> MDFGSLETVVANSAFIAARGSF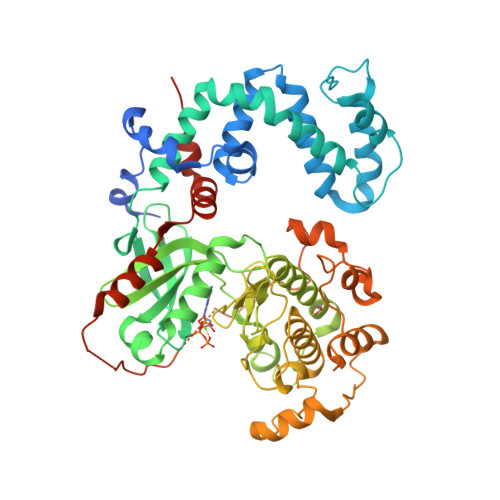DASSGPASRDRKYLARLKLPPLSKCEALRESLDLGFEGMCLEQPIGKRLFQQFLRTHEQHGPALQLWKDIEDYDTADDALRPQKAQALRAAYLEPQAQLFCSFLDAETVARARAGAGDGLFQPLLRAVLAHLGQAPFQEFLDSKYFLRFLQWKWLEAQPMGEDWFLDFRVLGRGGFGEVFACQMKATGKLYACKKLNKKRLKKRKGYQGAMVEKKILAKVHSRFIVSLAYAFETKTDLCLVMTIMNGGDIRYHIYNVDEDNPGFQEPRAIFYTAQIVSGLEHLHQRNIIYRDLKPENVLLDDDGNVRISDLGLAVELKAGQTKTKGYAGTPGFMAPELLLGEEYDFSVDYFALGVTLYEMIAARGPFRARGEKVENKELKQRVLEQAVTYPDKFSPASKDFCEALLQKDPEKRLGFRDGSCDGLRTHPLFRDISWRQLEAGMLTPPFVPDSRTVYAKNIQDVGAFSTVKGVAFEKADTEFFQEFASGTCPIPWQEEMIETGVFGDLNVWRPDGVDHHHHHH>[4x]MSLQRYFIELTKQQIEEAPTFSITGE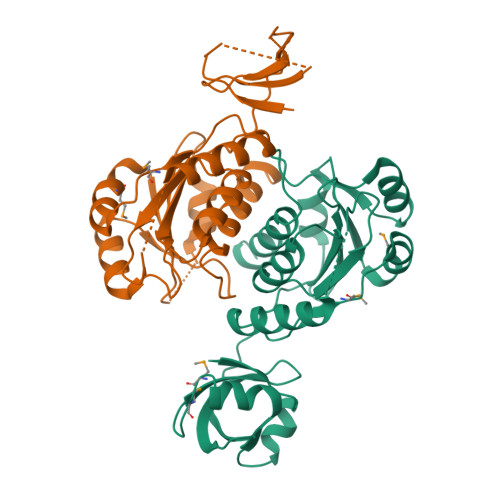EVHHIVNVMRMNEGDQIICCSQDGFEAKCELQSVSKDKVSCLVIEWTNENRELPIKVYIASGLPKGDKLEWIIQKGTELGAHAFIPFQAARSVVKLDDKKAKKKRERWTKIAKEAAEQSYRNEVPRVMDVHSFQQLLQRMQDFDKCVVAYEESSKQGEISAFSAIVSSLPKGSSLLIVFGPEGGLTEAEVERLTEQDGVTCGLGPRILRTETAPLYALSAISYQTELLRGDQEGGSHHHHHH>[4x]KSKTEYYNAWSEWERNAPPGNGEQREMAVSRLRDCLDRQAHELELNNLGLSSLPELPPHLERLVASCNSLTELPELPQSLKSLEVYENNLKALPDLPPLLVDLRVFNNQLEELPELQNLPFLTEIYANNNSLKTLPDLPPSLVDLNVRENYLTALPELPQSLIFLDISDNILSGLSELPPNLSCLDASRNGIRSLCDLPPSLVYLDVRDNQLIELPALPSGLERLIASFNHLAELPELPPNLYYLDASRNEISSLCDLPPSLVDLNVRKNQLIELPALPPDLERLIASFNHLAELPELPPNLSYLDASRNEISSLCDLPPSLVDLNVRKNQLIELPALPPDLERLIASFNHLAELPELPPNLSYLDASRNEISSLCDLPPSLVELDVRDNQLIELPALPPHLERLIASLNHLAEVPELPQNLKQLHVEHNALREFPDIPESVEDLRMD

Yersinia outer protein M (YopM) is a major virulence factor of the three pathogenic Yersinia species, Y. pestis, Y. pseudotuberculosis and Y. enterocolitica. Together with up to six other effector proteins YopM is translocated into host cells by the bacterial type three secretion apparatusand significantly contributes to the Yersinia infection strategy. The individual LRRs in YopM consist of 20- or 22 amino acids and together form a LRR-domain, which makes up the central and largest part of the protein. YopM isoforms of all three pathogenic Yersinia species were found to associate with the serine/threonine kinases RSK1 (p90 ribosomal S6 kinase 1; MAPKAP-K1) and PKN2 (protein kinase N2; protein kinase C related kinase2/PRK2).

The YopM_34–481 construct essentially consists of the LRR region and the two N-terminal α-helices that initiate LRR folding. The crystal structure revealed four molecules in the asymmetric unit. The asymmetric unit contains four molecules equivalent to two biological assemblies each represented by a dimer. Analysis of the interaction interfaces between the four YopM molecules indicated that two YopM molecules mutually interact by binding of the C-terminal LRR 20 (residues 461–481) of one molecule to the internal LRRs 14–17 (residues 342–422) of the other molecule. The total interface area comprises approximately 1010 Å2 and is mediated by 21 hydrogen bridges. The crystallographic dimer fitted the experimental SAXS data reasonably well (χ2 = 4.3), which could be further refined to a nearly perfect fit (χ2 = 2.3) by using a rigid body modelling to slightly change the angle between the two YopM molecules. Altogether these data indicate that a dimer represents the smallest biological assembly of YopM and that the dimer creates an interface that allows binding of one molecule of DDX3, thus forming a 2:1 YopM:DDX3 complex. It appears that the YopM dimer forms a binding interface for the DDX3 fragment. The first part of the binding interface covers an area of around 1000 Å2 and is formed by LRRs 7–9 of the first YopM molecule (green colored in Fig 3D). YopM's highly conserved unstructured C-terminal tail is not part of the previously published crystal structure or the novel crystal structure obtained in this work.> AKIGLFYGTQTGVTQTIAESIQQEFGGESIVDLNDIANADASDLNAYDYLIIGCPTWGVG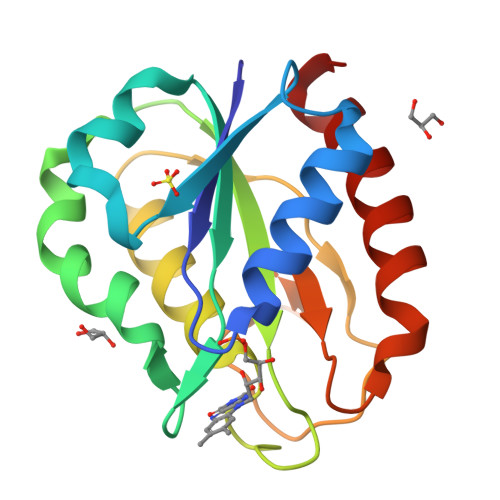ELQSDWEGIYDDLDSVNFQGKKVAYFGAGDQVGYSDNFQDAMGILEEKISSLGSQTVGYWPIEGYDFNESKAVRNNQFVGLAIDEDNQPDLTKNRIKTWVSQLKSEFGL>[4x]ENTMRALTLKDILNGTFSYKTFFPNWISGQEYLHQSADNNIVLYNIETGQSYTILSNRTMKSVNASNYGLSPDRQFVYLESDYSKLWRYSYTATYYIYDLSNGEFVRGNELPRPIQYLCWSPVGSKLAYVYQNNIYLKQRPGDPPFQITFNGRENKIFNGIPDWVYEEEMLATKYALWWSPNGKFLAYAEFNDTDIPVIAYSYYGDEQYPRTINIPYPKAGAKNPVVRIFIIDTTYPAYVGPQEVPV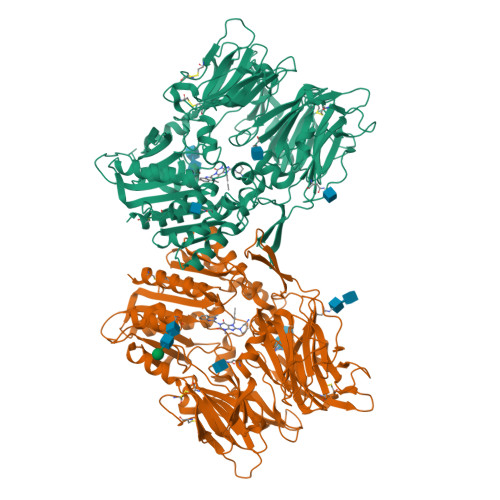PAMIASSDYYFSWLTWVTDERVCLQWLKRVQNVSVLSICDFREDWQTWDCPKTQEHIEESRTGWAGGFFVSTPVFSYDAISYYKIFSDKDGYKHIHYIKDTVENAIQITSGKWEAINIFRVTQDSLFYSSNEFEEYPGRRNIYRISIGSYPPSKKCVTCHLRKERCQYYTASFSDYAKYYALVCYGPGIPISTLHDGRTDQEIKILEENKELENALKNIQLPKEEIKKLEVDEITLWYKMILPPQFDRSKKYPLLIQVYGGPCSQSVRSVFAVNWISYLASKEGMVIALVDGRGTAFQGDKLLYAVYRKLGVYEVEDQITAVRKFIEMGFIDEKRIAIWGWSYGGYVSSLALASGTGLFKCGIAVAPVSSWEYYASVYTERFMGLPTKDDNLEHYKNSTVMARAEYFRNVDYLLIHGTADDNVHFQNSAQIAKALVNAQVDFQAMWYSDQNHGLSGLSTNHLYTHMTHFLKQCFS> SMSSTSPNLQKAIDLASKAAQEDKAGNYEEALQLYQHAVQ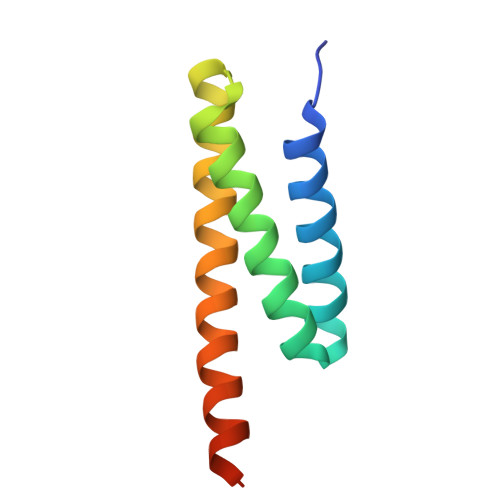YFLHVVKYEAQGDKAKQSIRAKCTEYLDRAEKLKEYLKNKEKKAQKPVKE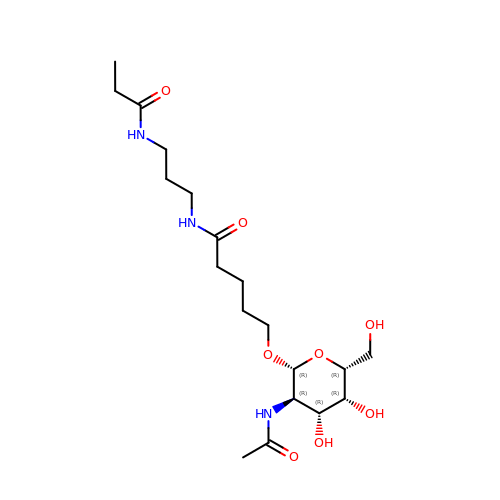5-[(2~{R},3~{R},4~{R},5~{R},6~{R})-3-acetamido-6-(hydroxymethyl)-4,5-bis(oxidanyl)oxan-2-yl]oxy-~{N}-[3-(propanoylamino)propyl]pentanamide | C19 H35 N3 O8 | IKUNNZGUTWUXRA-LQDZTQBFSA-N> MSLAKDVTIIYTNDLHAHVEPYKVPWIADGKRDIGGWANITTLVKQEKAKNKATWFFDAGDYFTGPYISSLTKGKAIIDIMNTMPFDAVTIGNHEFDHGWDNTLLQLSQAKFPIVQGNIFYQNSSKSFWDKPYTIIEKDGVKIG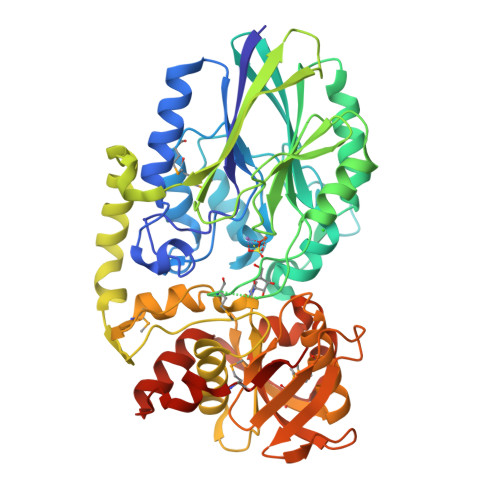VIGLHGVFAFNDTVSAATRVGIEARDEIKWLQRYIDELKGKVDLTVALIHEGVPARQSSMGGTDVRRALDKDIQTASQVKGLDILITGHAHVGTPEPIKVGNTLILSTDSGGIDVGKLVLDYKEKPHNFTVKNFELKTIYADEWKPDQQTKQVIDGWNKKLDEVVQQTVAQSPVELKRAYGESASLGNLAADALLAAAGKNTQLALTNSGGIRNEIPAGAITMGGVISTFPFPNELVTMELTGKQLRSLMEHGASLSNGVLQVSKGLEMKYDSSKPVGQRVITLTLNGKPIEDATVYHIATQSFLADGGDGFTAFTEGKARNITGGYYVYHAVVDYFKAGNTITDEQLNGMRVKDIKEGHHHHHH> GSVVIVGRINLSGDTAYAQQTRGEEGCQETSQTGRDKNQVEGEVQIVSTATQTFLATSINGVLWTVYHGAGTRTIASPKGPVTQMY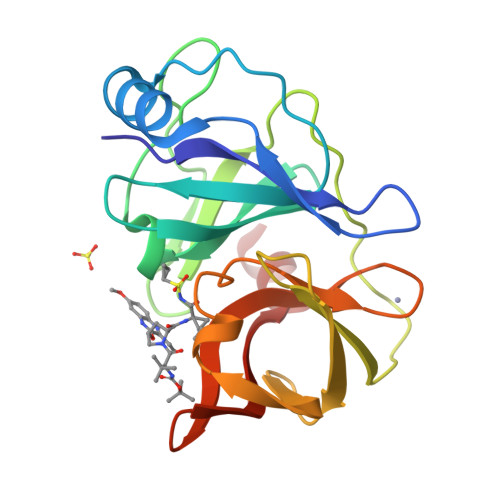TNVDKDLVGWQAPQGSRSLTPCTCGSSDLYLVTRHADVIPVRRRGDSRGSLLSPRPISYLKGSAGGPLLCPAGHAVGIFRAAVCTRGVAKAVDFIPVESLETTM> MWIQIVRFMSLIIDRFEMTKEQHVEFIRNLPDRDLYVEIDQDKITQVLDNIISNALKYSPEGGHVTFSIDVNEEEELLYISVKDEGIGIPKKDVEKVFDRFY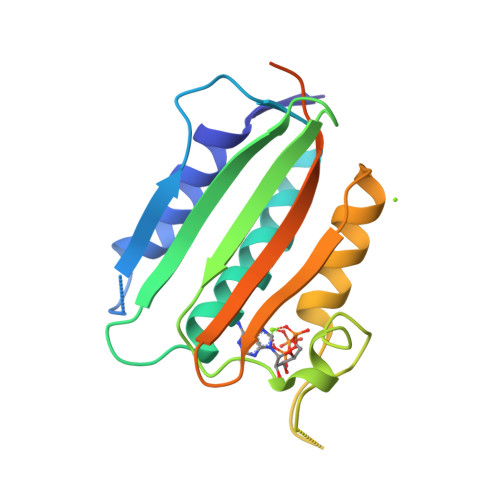RVDKARTRKLGGTGLGLAIAKEMVQAHGGDIWADSIEGKGTTITFTLPYKEEQEDDWDEAENLYFQSLEHHHHHH> MSF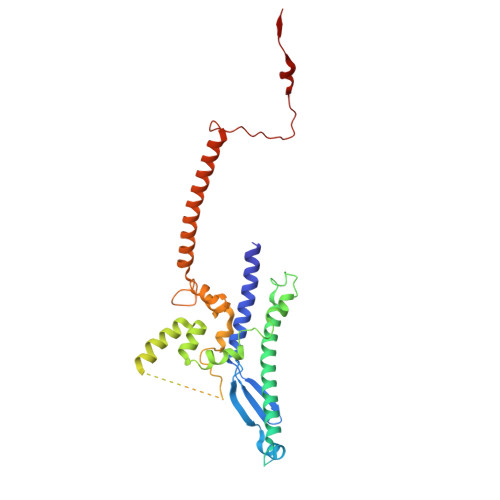RYTNNLIGALKHRLLLESSYREIASRKFIGNCRGVEVVCSGYGTVLAVQLTDKAVWESFYRKGGRPTVSGGGDVSGDAETGTQGSATTTGATGDLDLDKLAESIKTALWDATRKIRSAKEAALHRSLSHNTRMRASADLKHWYEEDANTLRPLAFEALKHEAATPWMQLVQHGKKEEAAALLKEFEQKGDAAEATPTRVKDDRVKGTRTELSNREQPPLASTLKAEDSNPATIPIGSVHPLFTPALVQIEEAGGGSVSNEAVCRAQLWELSRDEQLFWERVELIRKGQVASIGSSHKRGYADEAAFAKDDTEEKVQLRFTQ>MGSMTSDTARSYRFPEGFLWGAATAAYQIEGSSMADGAGESIWDRFSHTPGNMKDGDTGDVACDHYNRWREDIELMKRLNLQAYRFSVSWSRVIPQGRGAINPKGLAFYDRLVDGLLEAGIEPLATLYHWDLPAALDDRGGWLNPDIADWFADYGQVLFEKFKGRVKTWGTINQPWVIVDGGYLHGALAPGHRSAYEAVIAGHNVLRAHGAAVRRFREVGEGQIGIVLNIEPKYPASDKPEDEAARRRAEAQMNRWFLDPLMGRGYPEELTDVYGAAWREFPKEDFELIAEPTDWMGLNWYTRAVPENAPDAWPTRSRPVRQTQHAHTETGWEVYPPALTDTLVWLSEQTGGKLPLM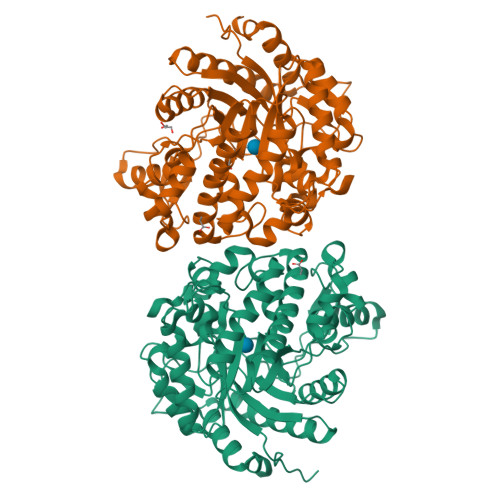VTENGSAWYDPPHAIDGRIHDPMRVHYLQTHIKALHDAIGKGVDLRGYMAWSLLDNLEWSLGYSKRFGIVHVNFATQERTIKDSGLLYAEVIKTHGDVLNTLKLHHHHHH[2x]FKRP recognizes RboP-(phospho-)core M3 as the RboP acceptor and transfers a RboP from CDP-Rbo to form the tandem RboP structure. Although FKRP exhibits RboP transferase, not NTase activity, our crystal structure clearly shows that FKRP belongs to the NTase superfamily as proposed previously. Our structural and biochemical analyses revealed the acceptor substrate recognition mechanism by dimer FKRP: the phosphate group of RboP is recognized by the catalytic domain of one subunit, and a phosphate group on O-mannose is recognized by the stem domain of another subunit. Indeed, mutations of FKRP, which is involved in synthesis of a tandem RboP structure, cause congenital muscular dystrophy;17–23 more than 15 missense mutations in the FKRP gene were found in LGMD2I (limb-girdle muscular dystrophy type 2I), MDDGB5 [muscular dystrophy-dystroglycanopathy (congenital with or without mental retardation, type B, 5)], and severe muscle-eye-brain disease/Walker-Warburg syndrome (MEB/WWS) patients (OMIM ID of FKRP; 606596).

To understand the molecular basis of the unique substrate recognition and catalytic reaction of FKRP, we determined the crystal structures of the sFKRP-CDP-Rbo complex with Ba2+ and the sFKRP-CMP complex with Mg2+ at 2.23 Å and 2.60 Å resolution, respectively. We tried to obtain the complex structure of sFKRP-CDP-Rbo with Mg2+ but could not. In the presence of Mg2+, electron densities could only be observed for the CMP moiety of CDP-Rbo; those for the RboP moiety were missing. Since FKRP is active with the Mg2+, CDP-Rbo would be catalyzed and only the CMP moiety would remain under the Mg2+-containing condition. The crystal structure of the sFKRP-CMP complex revealed a similarity of the metal ion coordination sites to those of NTase; one Mg2+ at site I coordinates Asp362 and Asp364, while the other Mg2+ at site II coordinates Asp362, Asp364, and Asp416. This similarity suggests that FKRP and NTase share a catalytic mechanism.

>[4x]GGRPAGPRVTVLVREFEAFDNAVPELVDSFLQQDPAQPVVVAADTLPYPPLALPRIPNVRLALLQPALDRPAAASRPETYVATEFVALVPDGARAEAPGLLERMVEALRAGSARLVAAPVATANPARCLALNVSLREWTARYGAAPAAPRCDALDGDAVVLLRARDLFNLSAPLARPVGTSLFLQTALRGWAVQLLDLTFAAARQPPLATAHARWKAEREGRARRAALLRALGIRLVSWEGGRLEWFGCNKETTRCFGTVVGDTPAYLYEERWTPPCCLRALRETARYVVGVLEAAGVRYWLEGGSLLGAARHGDIIPWDYDVDLGIYLEDVGNCEQLRGAEAGSVVDERGFVWEKAVEGDFFRVQYSESNHLHVDLWPFYPRNGVMTKDTWLDHRQDVEFPEHFLQPLVPLPFAGFVAQAPNNYRRFLELKFGPGVIENPQYPNPALLSLTGSG>MTYTVGHYLATRLAQIGLKHHFAVAGDYNLVLLDQLLKNKDLEQVYCCNELNCGFSAEGYARANGVGAAVVTFSVGALSAFNAIGGAYAENLPVILISGAPNTNDHGSGHILHHTIGTTDYGYQLEMAKQITCAAVSITHAEDAPALIDHAIRTALREKKPAYIEIACNVAAQPCARPGPVSALLNEPTSDEETLKAAVEAALDFIEKREKPVLLVGGKLRAAGAEEAVVELADALGCAVATMAAAKSFFPEDHPGYVGTYWGEVSSPGVEEIVDWADGIICLGPVFNDYSTVGWTAWPKGENVVLVDPHHITVGGEEFTGIHLKDFLTALTERVPKKDATLDQFKARVGKPAAE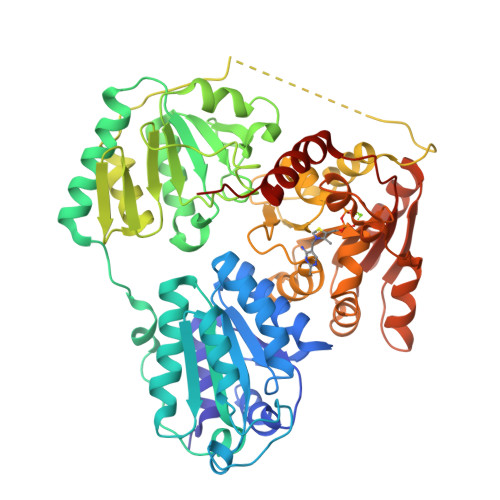KVPAADPNAPLTRAELCRQIQGLLNPNTTLIAETGDSWFNAMRMKLPHGARVELEMQWGHIGWSVPATFGYAVAEPERRNVLMVGDGSFQLTAQEVAQMVRRKLPIIIFLINNRGYTIEVKIHDGPYNNIKNWDYAGLMEVFNAEDGKGLGLKATTGGELAEAIKKALAHREGPTLIECVIDRDDCTPELVTWGKKVATANARPPQAI[4x]>[4x]GPSGMILKRAYDVTPQKISTDKVRGVRKRVLIGLKDAPNFVMRLFTVEPGGL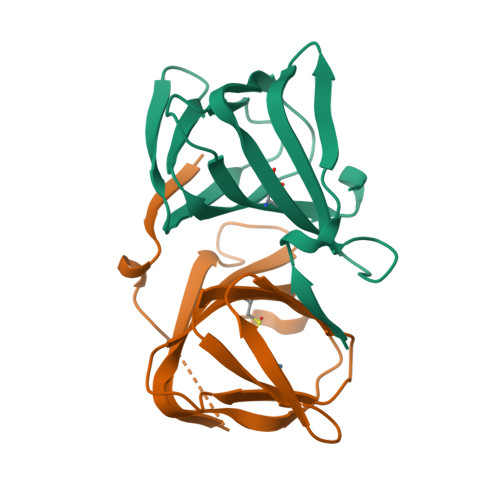IDRHSHPWEHEIFVLKGKLTVLKEQGEETVEEGFYIFVEPNEIHGFRNDTDSEVEFLCLIPKEGGE Quinabactin | C20 H24 N2 O3 S | 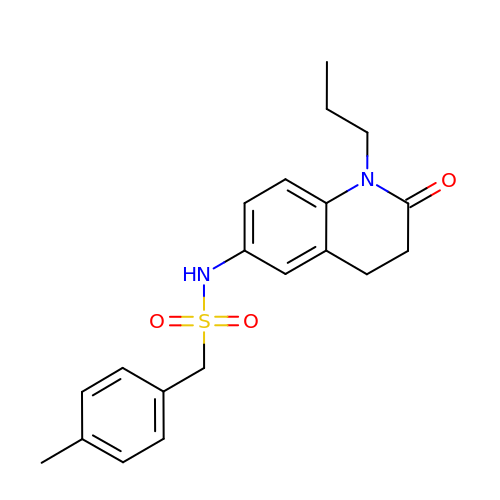IVHKSUMLZQXFPR-UHFFFAOYSA-N(2-{[2-(2-amino-6-oxo-1,6-dihydro-9H-purin-9-yl)ethyl](3-aminopropyl)amino}ethyl)phosphonic acid | C12 H22 N7 O4 P | 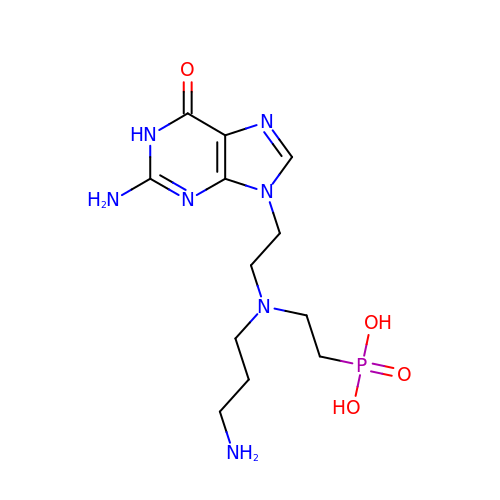JXSWXCFQTAYPAJ-UHFFFAOYSA-N> TPVSEKQLAEVVANTVTPLMKAQSVPGMAVAVIYQGKPHYYTFGKADIAANKPVTPQTLFELGSISKTFTGVLGGDAIARGEISLDDPVTRYWPQLTGKQWQGIRMLDLATYTAGGLPLQVPDEVTDNASLLRFYQNWQPQWKPGTTRLYANASIGLFGALAVKPSGMPYEQAMTTRVLKPLKLDHTWINVPKAEEAHYAWGYRDGKAVRAVRVSPGMLDAQAYGVKTNVQDMANWVMANMAPENVADASLKQGIALAQSRYWRIGSMYQGLGWEMLNWPVEANTVVEGSDSKVALAPLPVAEVNPPAPPVKASWVHKTGSTGGFGSYVAFIPEKQIGIVMLANTS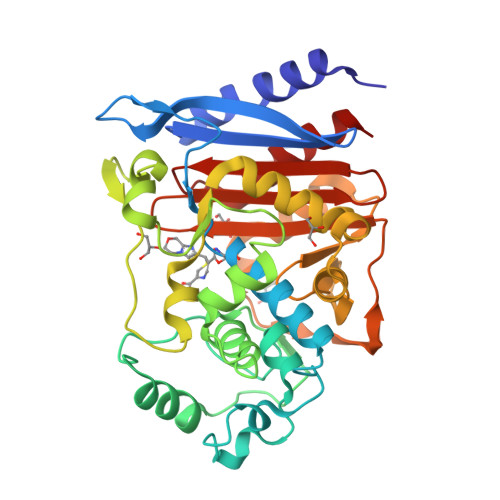YPNPARVEAAYHILEALQ N-[4-({[(3S)-oxolan-3-yl]methyl}carbamoyl)phenyl]-1,3-dihydro-2H-isoindole-2-carboxamide 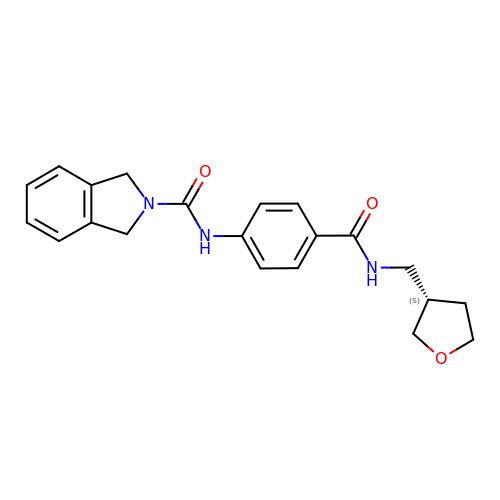| C21 H23 N3 O3 | BLZJCPAXCWJANZ-HNNXBMFYSA-N> MGSSHHHHHHSSPISPIETVPVKLKPGMDGPKVKQWPLTEEKIKALVEICTEMEKEGKISKIGPENPYNTPVFAIKKKDSTKWRKLVDFRELNKRTQDFWEVQLGIPHPAGLKKKKSVTVLDVGDAYFSVPLDEDFRKYTAFTIPSINNETPGIRYQYNVLPQGWKGSPAIFQSSMTKILEPFRKQNPDIVIYQYMDDLYVGSDLEIGQHRTKIEELRQHLLRWGLTTPDKKHQKEPPFLWMGYELHPDKWTVQPIVLPEKDSWTVNDICKLVGKLNWASQIYPGIKVRQLSKLLRGTKALTEVIPLTEEAELELAENREILKEPVHGVYYDPSKDLIAEIQKQGQGQWTYQIYQEPFKNLKTGKYARMRGAHTNDVKQLTEAVQKITTESIVIWGKTPKFKLPIQKETWETWWTEYWQATWIPEWEFVNTPPLVKLWYQLEKEPIVGAETFYVDGAANRETKLGKAGYVTNRGRQKVVTLTDTTNQKTELQAIYLALQDSGLEVNIVTDSQYALGIIQAQPDQSESELVNQIIEQLIKKEKVYLAWVPAHKGIGGNEQVDKLVSAGIRKVL;> PISPIETVPVKLKPGMDGPKVKQWPLTEEKIKALVEICTEMEKEGKISKIGPENPYNTPVFAIKKKDSTKWRKLVDFREL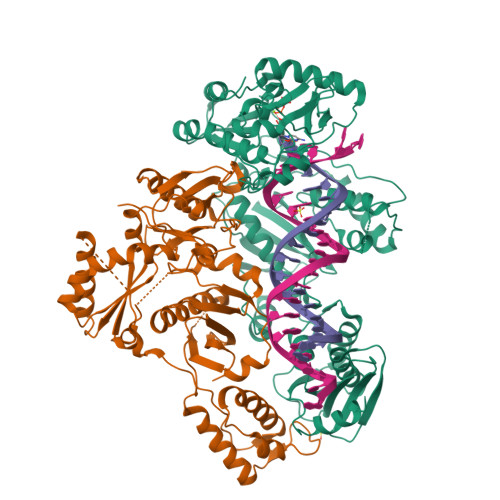NKRTQDFWEVQLGIPHPAGLKKKKSVTVLDVGDAYFSVPLDEDFRKYTAFTIPSINNETPGIRYQYNVLPQGWKGSPAIFQSSMTKILEPFRKQNPDIVIYQYMDDLYVGSDLEIGQHRTKIEELRQHLLRWGLTTPDKKHQKEPPFLWMGYELHPDKWTVQPIVLPEKDSWTVNDIQKLVGKLNWASQIYPGIKVRQLSKLLRGTKALTEVIPLTEEAELELAENREILKEPVHGVYYDPSKDLIAEIQKQGQGQWTYQIYQEPFKNLKTGKYARMRGAHTNDVKQLTEAVQKITTESIVIWGKTPKFKLPIQKETWETWWTEYWQATWIPEWEFVNTPPLVKLWYQLEKEPIVGAETF> GAGTSTPTTGNQNMSGNSGSIVQNFYMQQYQNSI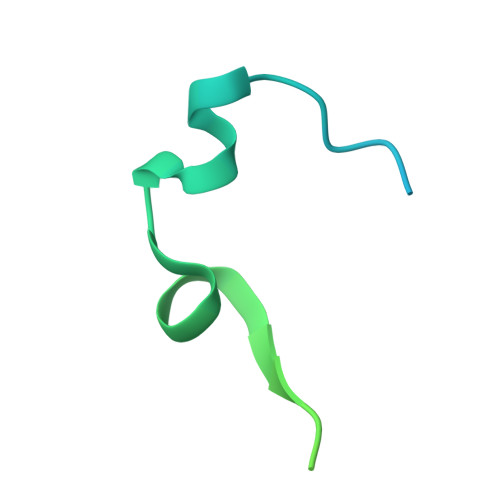DADLGDNVISPEGQGSNTSSSTSSSQSSGLGGWFSSLLNLGTKLLA> GPGSEFELMWLDMPSTAETGADQPAAGEVSDLLMLATPAATERVRREAEDIFRASSFRAGGAARRSEYRYAALAKDAYQQMGTAPVTEPP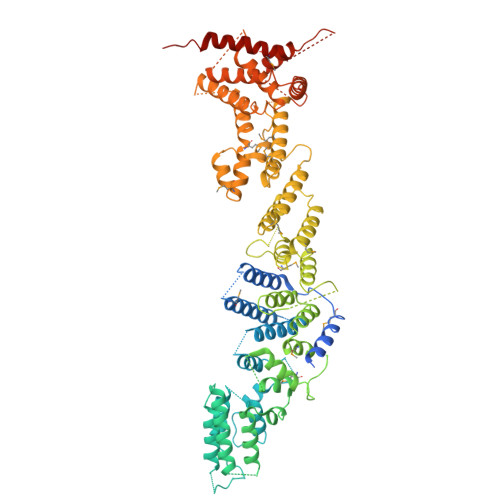QVILGTEDLLSRLYDEGVGEAEDEQKMDDTLATAAAQLAALWREHVDELPRPTEDHAAEIGPGPHATPFEKANYLANLALQIHHTRYEEGGLIRAEPLPQTLFRWLNEYHDMYGSQVDDILRHRPSPACHSLFWQAVFIALLRGKVGDAARLLDQAGWGHVRRGQRGEYAYVGQALENVQRAVDETIAVLESCPGFDGNWEIWSSDWTLFRVRARGLLEHLRRFAEGKDSAFGASAFSASAASAQSRQSMAGLARRAESQVPWEIYENLNIVFDIVLGQQGAILEAAQDWLEATVGLFGWWDERASRTEKPLSTSQSLSRSQALVLASAPANSESYLDRLARAFHTAVESDFHFNSQNAVEIGMACVFEDNIKGVIGLLRGWSLPIAAAVAEIASLGKWLPPHRPSGVYGLEDLDMDDLEVLGMDPGAPDEVDGIKDSTLVQYAQALADYEGLSSVQDRSGTSKDGWELSISVLGRMDSPERSEEMVRDLVEHLVQQLHVDSNATVDRLWFLLNELGMIEFAEDTTETYGDILARDSHRYGEAMWYYALAHRPNKVREVMNLLTSYSLIQSTAFPPANDLDDYLYKLLNDRKNTLEQCASQDMEAAELLGKMLSGYASLRQFYDIRDNEDALPHATPLSRRKQAATALISVIASSDDNIRGGLYDQTRDGIVSEDFLLALLGEALVFVSDPDNTNVHHGQLATPVITLDQIDVLLKAIEDLQAVGSRVYNACDEFLQLVLASAPGGLKGSTPADLLKKSAGPGPGGSGNAMLAGSSLVASQLQRSLSGTGGGLGKVAVKRRGWDWRSEVTAKTKGEDIMRRLRLGLAKDLAGLWLAEADEMVW> MASVHGTTYELLRRQGIDTVFGNPGSNELPFLKDFPEDFRYILALQEACVVGIADGYAQASRKPAFINLHSAAGTGNAMGALSNAWNSHSPLIVTAGQQTRAMIGVEALLTNVDAANLPRPLVKWSYEPASAAEVPHAMSRAIHMASMAPQGPVYLSVPYDDWDKDADPQSHHLFDRHVSSSVRLNDQDLDILVKALNSASNPAIVLGPDVDAANANADCVMLAERLKAPVWVAPSAPRCPFPTRHPCFRGLMPAGIAAISQLLEGHDVVLVIGAPVFRYHQYDPGQYLKPGTRLISVTCDPLEAARAPMGDAIVADIGAMASALANLVEESSRQLPTAAPEPAKVDQDAGRLHPETVFDTLNDMAPENAIYLNESTSTTAQMWQRLNMRNPGSYYFCAAGGEGFALPAAIGVQLAEPERQVIAVIGDGSANYSISALWTAAQYNIPTIFVIMNNGTYGALRWFAGVLEAENVPGLDVPGIDFRALAKGYGVQALKADN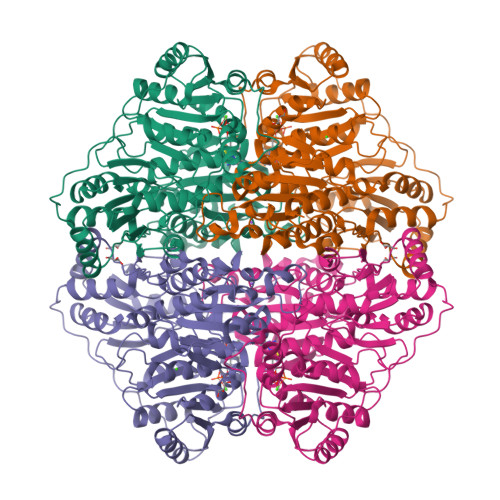LEQLKGSLQEALSAKGPVLIEVSTVSPVKRSHHHHHH>GQINVSFEFFPPRTSEMEQTLWNSIDRLSSLKPKFVSVTYGANSGERDRTHSIIKGIKDRTGLEAAPHLTCIDATPDELRTIARDYWNNGIRHIV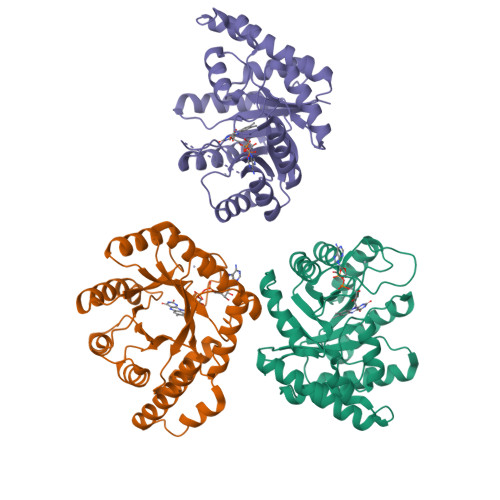ALRGDLPPGSGKPEMYASDLVTLLKEVADFDISVAAYPEVHPEAKSAQADLLNLKRKVDAGANRAITQFFFDVESYLRFRDRCVSAGIDVEIIPGILPVSNFKQAKKFADMTNVRIPAWMAQMFDGLDDDAETRKLVGANIAMDMVKILSREGVKDFHFYTLNRAEMSYAICHTLGVRPA[3x]> ACGGACAGCAGTCA;> CACACCGT;> CTGAC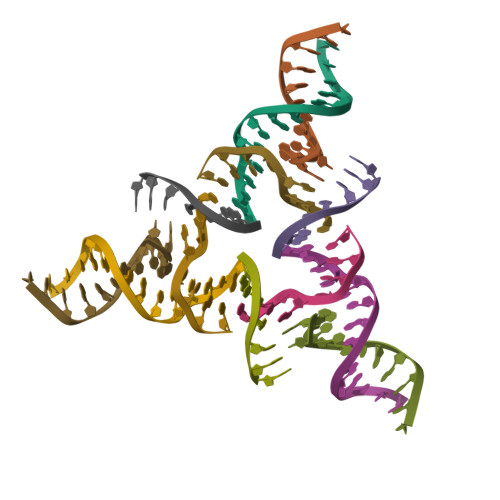TGCTGTGC;> GGCTGTG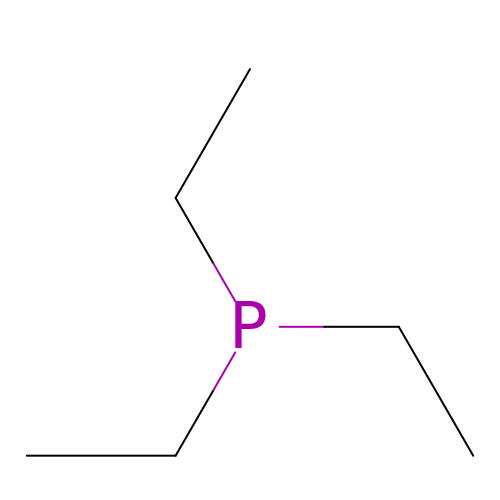TRIETHYLPHOSPHANE | C6 H15 P | RXJKFRMDXUJTEX-UHFFFAOYSA-N>[4x]MIQIYHADAFEIIKDFYQQNLKVDAIITDPPYNISVKNNFPTLKSAKRQGIDFGEWDKNFKLLEWIARYAPLVNPNGCMVIFCSYRFISYIADFLEENGFVVKDFIQWVKNNPMPRNIHRRYVQDTEFALWAVKKKAKWVFNKPKNEKYLRPLILKSPVVSGLEKTKHPTQKSLALMEKIISIHTNPNDIVLDPFMGSGTTGLACKNLERNFIGIESEKEYFQTAKKRLNLFLEHHHHHH

M1.HpyAVI is a DNA adenine MTase that belongs to the type II R-M system. M1.HpyAVI encoded by ORF hp0050 is an N6-adenine methyltransferase belonging to the β-class MTase. It has been reported recently that this enzyme recognizes the sequence of 5′-GAGG-3′, 5′-GGAG-3′ or 5′-GAAG-3′ and methylates adenines in these sequences. The structural basis and the catalytic mechanism underlying such a distinct activity are not well understood due to the lack of an available 3D structure of this enzyme.Here, we report the crystal structure of M1.HpyAVI from H. pylori 26695, which is the first determined N6-adenine MTase structure in H. pylori.

The cofactor-free and AdoMet-bound proteins were crystallized at different conditions. Both structures were determined by means of molecular replacement, and refined to 3.0 Å and 3.1 Å, respectively. Four and eight protein monomers resided in the asymmetric units of the two crystal structures. The two structures are very similar to each other and could be well overlaid with an RMSD of 0.76 Å on 191 Cα atoms. Some amino acids, particularly those within two loops (residues 32-61 and 152-172) in both structures, were poorly defined in electron density and had to be omitted from the refined models. The overall architecture of M1.HpyAVI revealed in these structures resembles the AdoMet-dependent MTase fold in which a twisted seven-stranded β-sheet flanked by six α-helices forms the structural core. In agreement, a dimer of M1.HpyAVI was observed in our crystal structures with the two monomers related by a two-fold axis. An area of ~1900 Å2 was buried at the dimeric interface, taking up ca 17% of the total area. Another difference locates at the highly flexible loop between β4 and αD (residues 33-58) of M1.HpyAVI, which was invisible in our structures but present in the structures of M.MboIIA and M.RsrI. Collectively, M1.HpyAVI possesses a long disordered TRD, which is in sharp contrast to the secondary structure-rich TRD in other β-class N6 adenine or N4 cytosine MTases or the extra DNA binding domain present in DNA MTases from other subgroups.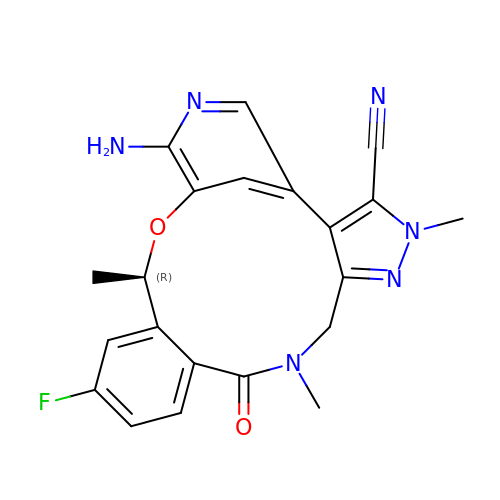(10R)-7-amino-12-fluoro-2,10,16-trimethyl-15-oxo-10,15,16,17-tetrahydro-2H-8,4-(metheno)pyrazolo[4,3-h][2,5,11]benzoxadiazacyclotetradecine-3-carbonitrile | C21 H19 F N6 O2 | IIXWYSCJSQVBQM-LLVKDONJSA-N>GGCG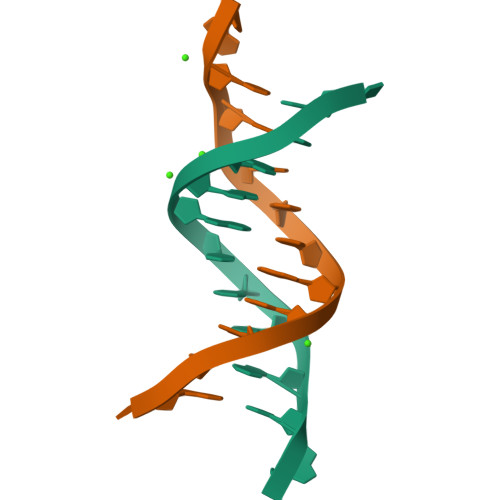AATTCGCG[2x]(4R)-4-oxidanyl-2-oxidanylidene-heptanedioic acid | C7 H10 O6 | 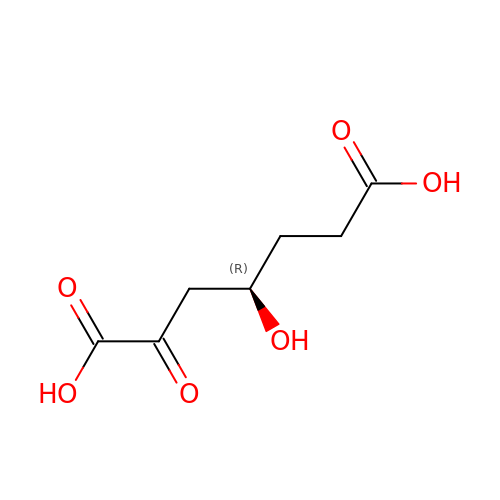HNOAJOYERZTSNK-SCSAIBSYSA-N>GSNEIKRGAVDLIKTGVNEKAMAGAVFSLFKKDGTEVKKELATDANGHIRVQGLEYGEYYFQETKAPKGYVIDPTKREFFVKNSGTINEDGTITSGTVVKMEVKNNEEPTIDKKINGKLEALPINPLTNYNYDIKTLIPEDIKEYKKYVVTDTLDNRLVIQGKPIVKIDGAEVNANVVEVAIEGQKVTATVKDFTKMDGKKEFHLQIKSQVKEGVPSGSEILNTAKIHFTNKNDVIGEKESKPVVVIPTTGIIELTKIDSANKNKMKGAEFVLKDNNGKIVVVAGKEVTGVSDENGVIKWSNIPYGDYQIFETKAPTYTKEDGTKTSYQLLKDPIDVKISENNQTVKLTIE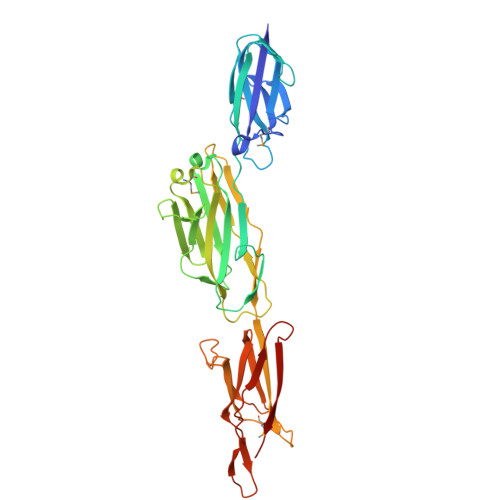NNKS[2x]> GPNLFVALYDFVASGDNTLSITKGEKLRVLNNTENGEWCEAQTKNGQGWVPSNYITPVN

The Src homology 3 (SH3) domain is a ∼60-residue modular domain that consists of two antiparallel β-sheets orthogonally packed to form a single hydrophobic core. This domain is present in many proteins and regulates critical cellular pathways by recognizing polyproline-rich motifs (PRMs; Kurochkina & Guha, 2013). Three-dimensional domain swapping (3D-DS) is a mechanism by which some proteins can oligomerize by exchanging identical domains or structural elements between monomers. In previous work, the 3D-DS of the c-Src SH3 domain has been characterized and its dependence on experimental conditions has been described. This work explores the role of the hinge-loop composition by interchanging residues in the RT and n-Src loops between two SH3 domains: one being the c-Src SH3 domain, where 3D-DS has been described, and the other being the Abl SH3 domain, where 3D-DS has not been described to date.

However, the interchange of one or two loops within the Abl SH3 domain produces a noticeable reduction in its stability but does not promote the formation of 3D domain-swapped oligomers. Conversely, replacing the RT and n-Src loop residues in the Abl_Src chimeras with those from the c-Src SH3 domain results in destabilization under identical denaturing conditions. Notably, the Abl_Src-nSrc and Abl_Src-2 chimeras exhibit pronounced destabilization, highlighting a key role for the c-Src n-Src loop residues in determining the stability of these chimeric proteins. Meanwhile, the Abl_Src chimeras showed lower Tm values than the WT protein, and the chimeras most affected by the exchange of the loops are those where the n-Src loop of the c-Src was introduced. In this way, the ΔG values are the same for the WT and Abl_Src-RT, but the Abl_Src-nSrc and Abl_Src-2 chimeras show a noticeable loss of stability. Although the conformation is slightly different in the RT loop, the hydrogen bonds are conserved. In the n-Src loop, there are significant differences between the WT protein and Abl_Src-nSrc, but also with the Abl_Src-RT and Abl_Src-2 chimeras. However, Src_Abl-nSrc shows an ordered distal loop in most of the molecules in the asymmetric unit and this chimera does not form the intertwined dimer. The same behaviour can be observed in the Abl_Src chimeras, where the distal loop shows low B factors. Indeed, even though the Abl_Src chimeras are less stable, this reduction in stability does not allow formation of the intertwined dimer. Meanwhile, the behaviour is the opposite in the Abl_Src chimeras, and the Abl_Src-n-Src chimera shows higher solubility than the Abl_Src-RT and Scr_Abl-2 chimeras.> MSEIGTSFPFDPHYVEVLGSRMHYVDVGPRDGTPVLFLHGNPTSSYLWRNIIPHVAPTHRCIAPDLIGMGKSDKPDLDYRFEDHVRYLDAFIEALGLEDVVLVIHDWGSALGFHWARRNPERVRGIAFMEFIRPIPTWDEWPEFARELFKAFRTPGVGRKMIIEQNMFIEQILPAFVVRPLTEEEMDHYREPFLKPEWREPLWRFPNELPIAGEPADVWALVEAYMRWLHQSPVPKLLFWGEPGVLIPPEEAERCRESLPNLKTVFIGPGLHYLQEDNPDEIGSEIARWLPALHHHHHH

The target protein used in this study is the computationally stabilized haloalkane dehalogenase DhaA115 designed previously using the web server FireProt. Eleven mutations that were originally introduced in the wild type increased its apparent melting temperature (Tmapp) to approx. 73 °C (ΔTmapp ∼ 23 °C), making it the most stable haloalkane dehalogenase to date. First, DhaA115 displays activity toward a broad range of halogenated substrates, many of which are toxic and carcinogenic compounds persistent in the environment, e.g., 1,2-dichloroethane and 1,2-dibromoethane. This makes the enzyme particularly valuable for biotechnological applications that detoxify and degrade harmful pollutants.

Moreover, the removal of 3 mutations possessing a low probability of substitution (D11P, A212D, and L221I) from DhaA222 resulted in a further increase of thermostability by 1 °C (DhaA231). The analysis supported our conclusions about the disruptive mutations and, more importantly, succeeded in identifying three additional false positives, as demonstrated by the improved stability of DhaA231. We obtained diffraction-quality crystals of DhaA223 and DhaA231 enzymes that belonged to the space groups P1211 and P212121 and diffracted at 1.5 and 1.3 Å resolution, respectively. The positioning of catalytic pentad residues was not disturbed, which is a prerequisite for efficient catalysis. Here, we show that the protein backbones of DhaA223 and DhaA231 superpose well with that of the DhaA115, although some minor changes are observed in the hinge regions between the helical cap domain and the hydrolase core. The crystal structures of DhaA223 and DhaA231 thus suggest that stabilization was achieved via strengthening intricate networks of residue-to-residue interactions, stabilizing the αβα-sandwich architecture. The resistance to urea-induced denaturation increased in the order of DhaA115 < DhaA222 < DhaA223 < DhaA231 and the best fit in all four cases was achieved using the three-state model of unfolding (black lines). We show that the mutations designed by FireProt and PROSS stabilized the native state of DhaA115 and increased the unfolding energy barrier, shifting their maximal activity temperatures above 65 °C. We also observe that the stabilization of DhaA is accompanied by the destabilization of an intermediate state based on the increasing cooperativity of unfolding (most noticeably for DhaA231). The increased turnovers of DhaA222 and DhaA231 stem from a decrease in the transition state’s energy barrier (7 and 6 kJ/mol, respectively).>MHPGFFTSIGQMTDLIHTEKDLVTSLKDYIKAEEDKLEQIKKWAEKLDRLTSTATKDPEGFVGHPVNAFKLMKRLNTEWSELENLVLKDMSDGFISNLTIQRQYFPNDEDQVGAAKALLRLQDTYNLDTDTISKGNLPGVKHKSFLTAEDCFELGKV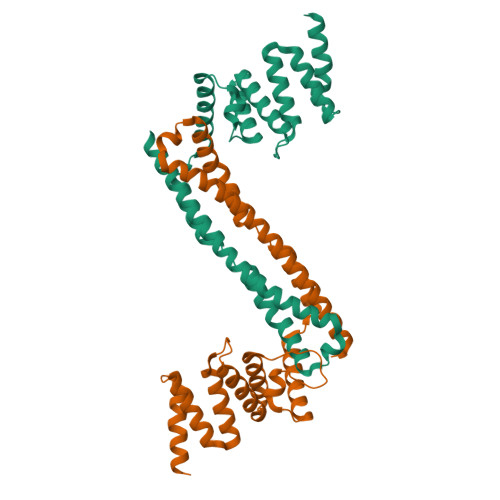AYTEADYYHTELWMEQALRQLDEGEISTIDKVSVLDYLSYAVYQQGDLDKALLLTKKLLELDPEHQRANGNLKYFEYIMAKE[2x]> GSHMGVTVERIAPGDGKNFPKKGDKVTIHYVGTLENGDKFDSSRDRGSPFQCT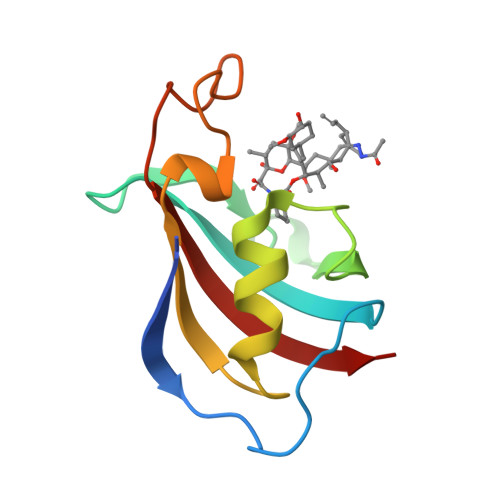IGVGQVIKGWDEGVTQLSVGEKARLICTHDYAYGERGYPGLIPPKATLNFEVELIKIN5-AMINO-1H-[1,2,3]TRIAZOLO[4,5-D]PYRIMIDIN-7-OL 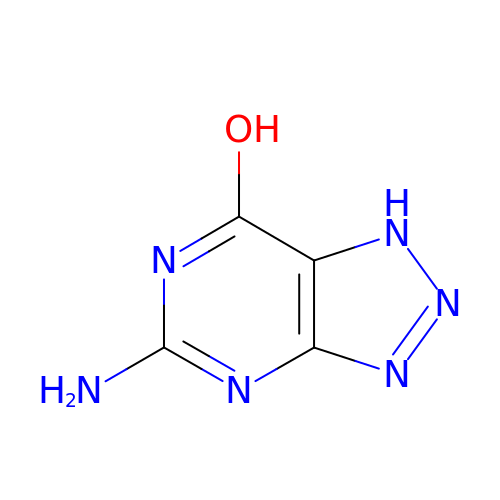| C4 H4 N6 O | LPXQRXLUHJKZIE-UHFFFAOYSA-N> GKITFYEDRGFQGHCYECSSDCPNLQPYFSRCNSIRVDSGCWMLYERPNYQGHQYFLRRGDYPDYQQWMGFNDSIRSCRLIPQHTGTFRMRIYERDDFRGQMSEITDDCPSLQDRFHLTEVHSL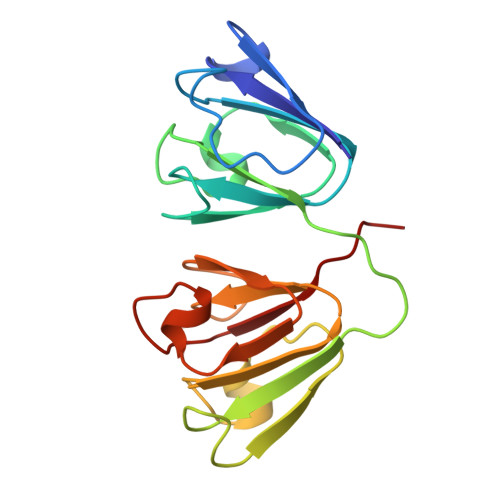NVLEGSWVLYEMPSYRGRQYLLRPGEYRRYLDWGAMNAKVGSLRRVMDFY>MMCLKLNLLDHVFANPFMNAAGVLCCTEEDLRCMTASSSGALVSKSCTSAPRDGNPEPRYMAFPLGSINSMGL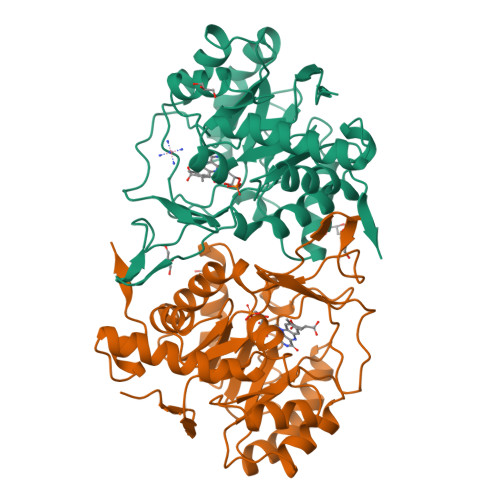PNLGFDFYLKYASDLHDYSKKPLFLSISGLSVEENVAMVRRLAPVAQEKGVLLELNLSCPNVPGKPQVAYDFEAMRTYLQQVSLAYGLPFGVKMPPYFDIAHFDTAAAVLNEFPLVKFVTCVNSVGNGLVIDAESESVVIKPKQGFGGLGGKYILPTALANVNAFYRRCPDKLVFGCGGVYSGEDAFLHILAGASMVQVGTALQEEGPGIFTRLEDELLEIMARKGYRTLEEFRGRVKTIE[2x]> LVPGEEWEFEVTAFYRGRQVFQQTISCPEGLRLVGSEVGDRTLPGWPVTLPDPGMS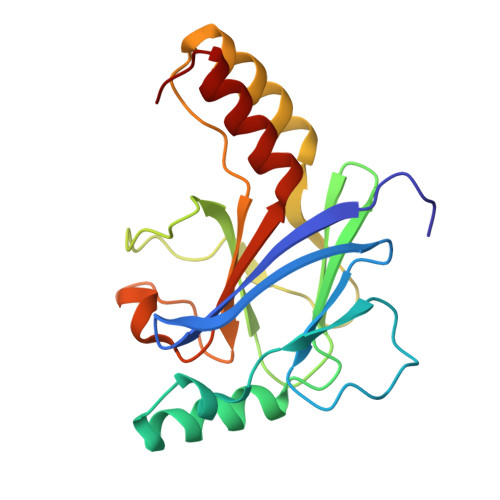LTDRGVMSYVRHVLSCLGGGLALWRAGQWLWAQRLGHCHTYWAVSEELLPNSGHGPDGEVPKDKEGGVFDLGPFIVDLITFTEGSGRSPRYALWFCVGESWPQDQPWTKRLVMVKVVPTCLRALVEMARVGGASS> APGVTVTPATGLSNGQTVTVSATGLTPGTVYHVGQCAVVEPGVIGCDATTSTDVTADAAGKITAQLKVHSSFQAVVGAD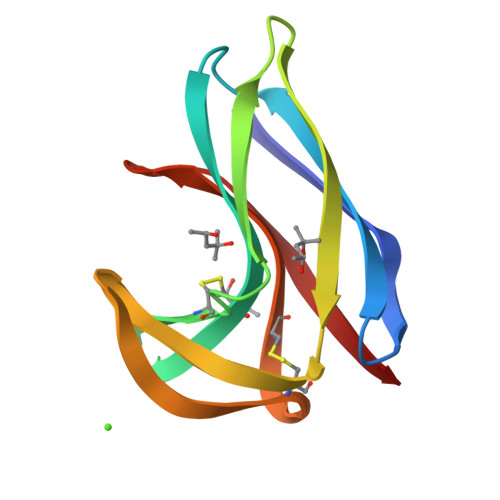GTPWGTVNCKVVSCSAGLGSDSGEGAAQAITFA NadR belongs to the MarR (Multiple Antibiotic Resistance Regulator) family, a group of ligand-responsive transcriptional regulators ubiquitous in bacteria and archaea. NadR binds the nadA promoter and represses gene transcription. In the presence of 4-hydroxyphenylacetate (4-HPA), a catabolite present in human saliva both under physiological conditions and during bacterial infection, the binding of NadR to the nadA promoter is attenuated and nadA expression is induced. Each NadR monomer consists of six α-helices and two short β-strands, with helices α1, α5, and α6 forming the dimer interface.

First, we crystallized NadR (a selenomethionine-labelled derivative) in the presence of a 200-fold molar excess of 4-HPA. The NadR/4-HPA structure revealed the ligand-binding site nestled between the dimerization and DNA-binding domains. Unexpectedly, only one monomer of the holo-NadR homodimer contained 4-HPA in the binding pocket, whereas the corresponding pocket of the other monomer was unoccupied by ligand, despite the large excess of 4-HPA used in the crystallization conditions. Inspection of the protein-ligand interaction network revealed no bonds from NadR backbone groups to the ligand, but several key side chain mediated hydrogen (H)-bonds and ionic interactions, most notably between the carboxylate group of 4-HPA and Ser9 of chain A (SerA9), and chain B residues TrpB39, ArgB43 and TyrB115. At the other ‘end’ of the ligand, the 4-hydroxyl group was proximal to AspB36, with which it may establish an H-bond (see bond distances in Table 3). In addition to the H-bonds involving the carboxylate and hydroxyl groups of 4-HPA, binding of the phenyl moiety appeared to be stabilized by several van der Waals’ contacts, particularly those involving the hydrophobic side chain atoms of LeuB21, MetB22, PheB25, LeuB29 and ValB111. Specifically, upon analysis with the CASTp software, the pocket in chain B containing the 4-HPA exhibited a total volume of approximately 370 Å3, while the pocket in chain A was occupied by these three side chains that adopted ‘inward’ positions and thereby divided the space into a few much smaller pockets, each with volume < 50 Å3, evidently rendering chain A unfavorable for ligand binding. Taken together, these observations suggest that Arg43 is a major determinant of ligand binding, and that its ‘inward’ position inhibits the binding of 4-HPA to the empty pocket of holo-NadR. Specifically, in addition to the different inter-helical translational distances, the α4 helices in the holo-NadR homodimer were also reoriented, resulting in movement of α4 out of the major groove, by up to 8Å, and presumably preventing efficient DNA binding in the presence of 4-HPA. Subsequently, upon ligand binding, holo-NadR adopts a structure less suited for DNA-binding and this conformation is selected and stabilized by a network of protein-ligand interactions and concomitant rearrangements at the NadR holo dimer interface.

>[2x]MPTQSKHASINIGLIQAREALMTQFRPILNQANITDQQWRIIRLLAENGTLDFQDLANQACILRPSLTGILTRLEKAGLVVRLKPSNDQRRVFLKLTAEGEKLYEEIGEEVDERYDAIEEVLGREKMLLLKDLLAELAKIEDALNS>MQSATQGKETATTTSSGTTYYVSSAHGDDANAGTSENAPWKSLTKVNDIASDLGPGDSVLLEYGSEFNDQYLHIKDTAGNADAPITISAYGDADEGKPVIASNGVKGSQWEQDYRANVGNHKNKGTVSTTLLLKDVSYITVSNLEITNDDADVYDPIDTWKWTDTPDSDGTKLDRSASRMDRTGVAGIAENGATMSNVTLDNLYIHDVDGNIYNKHMANGGIYFMAHYPMENTSAETDVWLREHVSRFDHVTIRNSTVKDVDRWGIAVGYTAYLNYIDANYGDGSIDDALIAKYGSTNVRIENNYVKGAGGDAITLMYCD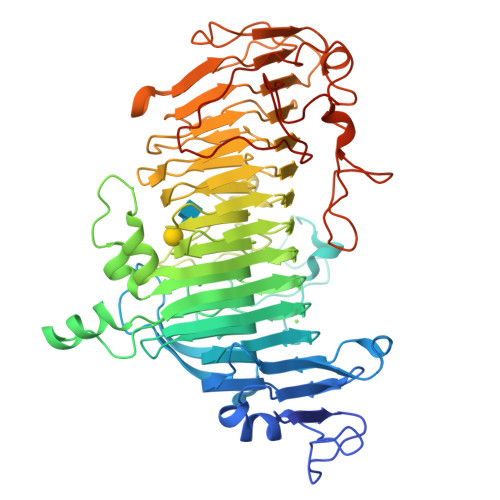RPVIEHNVGDSVSKHINTQDYTQPGSYGGRVAAGIWPWRCKDPVFQYNEMYNNLNAEHGNGDGQAWDADYGDGTLYQYNYSYGNSFASLMICNWYAVNTTFRYNISQNDRQGVFDLPSNGPGNHIYNNTVYVDADSQVLTKRSNSQSLFENNIFINATNTKKTETWNRGSQNGGQTYDNNMYVNYANKPTSDANAIEADDVSAVLAGAGSAPTSALKSGAEHARTGEKAAFDGYRPVAGSKAINAGKVVSDLNDYAVENDFLGNAVKGRPDLGAVEAALEHHHHHH[2x]>MGSSHHHHHHENLYFQGSMEQAIINDEREYLRHFWHPVCTVTELEKAHPSSLGPLAVKLLNEQLVVAKLGDEYVAMRDRCAHRSAKLSLGTVSGNRLQCPYHGWQYDTHGACQLVPACPNSPIPNKAKVDRFDCEERYGLIWIRLDSSFDCTEIPYFSAANDPRLRIVIQEPYWWDATAERRWENFTDFSHFAFIHPGTLFDPNNAEPPIVPMDRFNGQFRFVYDTPEDMAVPNQAPIGSFSYTCSMPFAINLEVSKYSSSSLHVLFNVSCPVDSHTTKNFLIFAREQSDDSDYLHIAFNDLV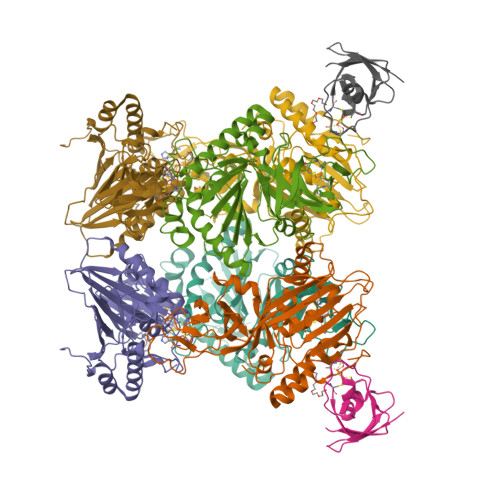FAEDKPVIESQWPKDAPADEVSVVADKVSIQYRKWLRELKEAHKEGSQAFRSALLDPVIESDRSYI[3x];> EYEVELKKTGQIFTVSPGSTLLQACLDNDVRIEASCEQGVCGTCITPVVSGDLEHHDTYLSKKERESGKWIMPCVSRCKSKKIVLDL> GHMLQNNTDYPFEANNPYMYHENPMEEGLSMLKLANLAEAALAFEAVCQAAPEREEAWRSLGLTQAENEKDGLAIIALNHARMLDPKDIAVHAALAVSHTNE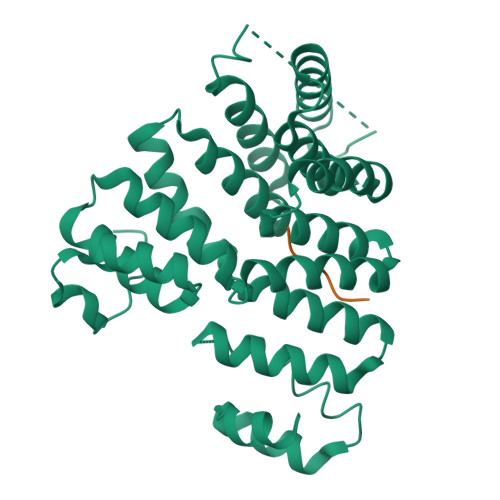HNANAALASLRAWLLSQPQYEQLGSVNLQADVDIDDLNVQSEDFFFAAPNEYRECRTLLHAALEMNPNDAQLHASLGVLYNLSNNYDSAAANLRRAVELRPDDAQLWNKLGATLANGNRPQEALDAYNRALDINPGYVRVMYNMAVSYSNMSQYDLAAKQLVRAIYMQVGGTTPTGEASREATRSMWDFFRMLLNVMNRPDLVELTYAQNVEPFAKEFGLQSMLL;> GTLSNRASKL>[2x]CPRFLKVKNWETDVVLTDTLHLKSTLETGCTEHICMGSIMLPSQHTRKPEDVRTKDQLFPLAKEFLDQYYSSIKRFGSKAHMDRLEEVNKEIESTSTYQLKDTELIYGAKHAWRNASRCVGRIQWSKLQVFDARDCTTAHGMFNYICNHVKYATNKGNLRSAITIFPQRTDGKHDFRVWNSQLIRYAGYKQPDGSTLGDPANVQFTEICIQQGWKAPRGRFDVLPLLLQANGNDPELFQIPPELVLE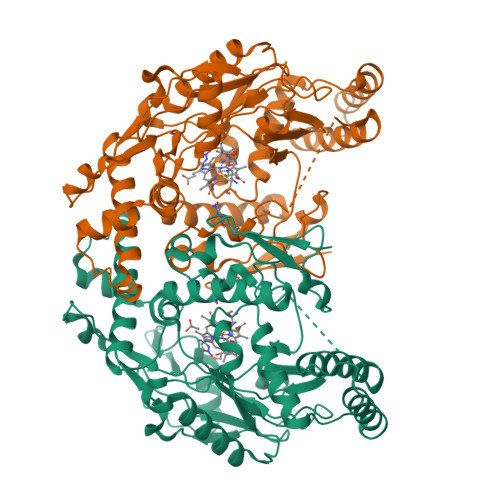VPIRHPKFDWFKDLGLKWYGLPAVSNMLLEIGGLEFSACPFSGWYMGTEIGVRNYCDNSRYNILEEVAKKMDLDMRKTSSLWKDQALVEINIAVLYSFQSDKVTIVDHHSATESFIKHMENEYRCRGGCPADWVWIVPPMSGSITPVFHQEMLNYRLTPSFEYQPDPWNTHVWK>GSVGPGLLGVSTLGPKRNSMVLDVAFVLEGSDKIGEADFNRSKEFMEEVIQRMDVGQDSIHVTVLQYSYMVTVEYPFSEAQSKGDILQRLREIRYQGGNRTNTGLALRYLSDHSFLVSQGDREQAPNLVYMVTGNPASDEIKRLPGDIQVVPIGVGPNANVQE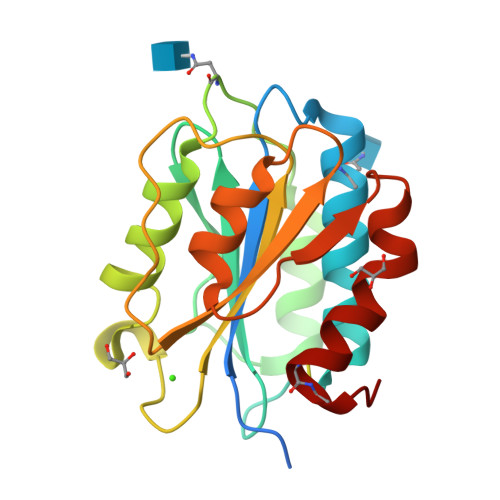LERIGWPNAPILIQDFETLPREAPDLVLQRCCSGEG[3x]> MTEETITIDSISNGILNNLLTTLIQDIVARETTQQ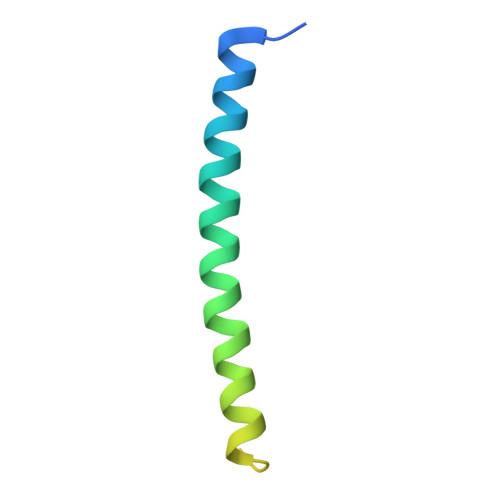QLLKTRYPDLRSYYFDPNGSLDINGLQKQQESSQYIH> MLPRETDEEPEEPGRRGSFVEMVDNLRGKSGQGYYVEMTVGSPPQTLNILV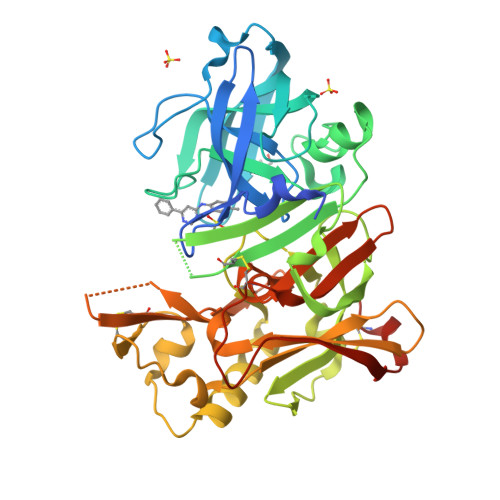DTGSSNFAVGAAPHPFLHRYYQRQLSSTYRDLRKGVYVPYTQGAWAGELGTDLVSIPHGPNVTVRANIAAITESDKFFINGSNWEGILGLAYAEIARPDDSLEPFFDSLVKQTHVPNLFSLQLCGAGFPLNQSEVLASVGGSMIIGGIDHSLYTGSLWYTPIRREWYYEVIIVRVEINGQDLKMDCKEYNYDKSIVDSGTTNLRLPKKVFEAAVKSIKAASSTEKFPDGFWLGEQLVCWQAGTTPWNIFPVISLYLMGEVTNQSFRITILPQQYLRPVEDVATSQDDCYKFAISQSSTGTVMGAVIMEGFYVVFDRARKRIGFAVSACHVHDEFRTAAVEGPFVTLDMEDCGYNIPQTDEST> MSQPSTANGGFPSVVVTAVTATTSISPDIESTWKGLLAGESGIHALEDEFVTKWDLAVKIGGHLKDPVDSHMGRLDMRRMSYVQRMGKLLGGQLWESAGSPEVDPDRFAVVVGTGLGGAERIVESYDLMNAGGPRKVSPLAVQMIMPNGAAAVIGLQLGARAGVMTPVSACSSGSEAIAHAWRQIVMGDADVAVCGGVEGPIEALPIAAFSMM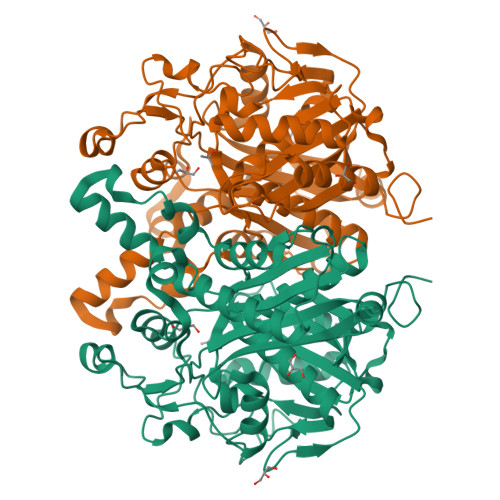RAMSTRNDEPERASRPFDKDRDGFVFGEAGALMLIETEEHAKARGAKPLARLLGAGITSDAFHMVAPAADGVRAGRAMTRSLELAGLSPADIDHVNAHGTATPIGDAAEANAIRVAGCDQAAVYAPKSALGHSIGAVGALESVLTVLTLRDGVIPPTLNYETPDPEIDLDVVAGEPRYGDYRYAVNNSFGFGGHNVALAFGRY> AUSAEQVEKLRNKINNAAVLVFAKSFCPYCKKVMERFNNLKIPFGYLDLDLKKNGSDYQKMLQEITGRTTVPQVFFRGEFIGGCDDVMAIDDDTIVKKANEMKYDYDMVIIGGGSGGLALAKESAKSGAKVALLDFVVPTPMGTTWGLGGTCVNVGCIPKKLMHQAALLNHYMEDAKSFGWDVDKGPHDWVKMVEGIQDHIHALNFGYRSSMMNANVKYLNALGEIVDPHTIKTTNKQGIVKNITTNTIIVATGERPRYPPIPGAKEYGITSDDLFTLDHNPGKTLCVGASYVSLECAGFLSSIGCDVTVMVRSIFLRGFDQQMAGLISDYIAKYGVKFVRPCVPTSVRCLEEYDPESGKLAIYEVEGKHEDGTPFKDTFNTVLFAVGRDPCTTNIGLQNVDVKTTNGRVVVDDEERTNVPNIYAIGDVSNAGYQLTPLAIQAGKNLARRLYTADDCRTDYTNVPTTVFTPLEYGCIGLSEENAISKFGEDNI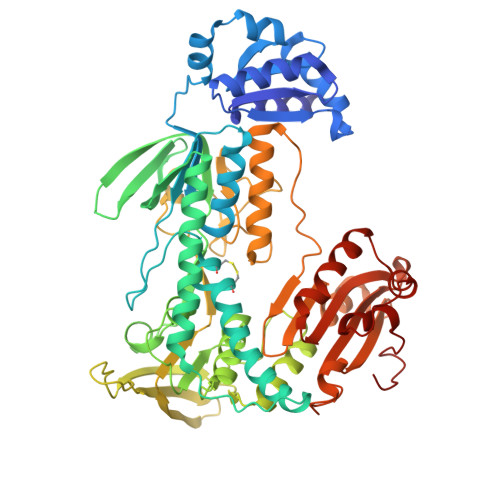EVFHSYFQPLEWTVPHRPDNTCYAKLIINKQDDNRVVGFHVFGPNAGEVTQGYAVAMHLGARKEDFDRTIGIHPTCSETFTTLRVTKSSGASA9-phenyl-4H-imidazo[1,2-a]indeno[1,2-e]pyrazin-4-one | C19 H11 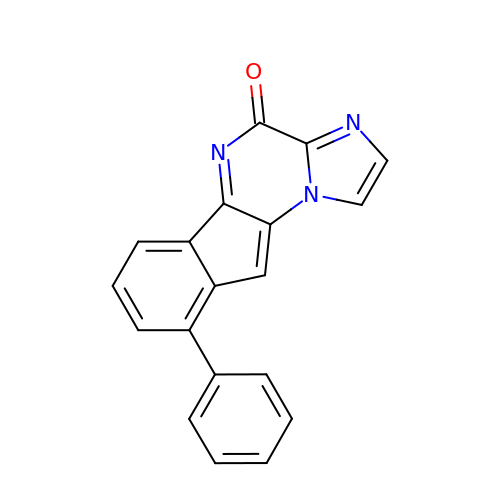N3 O | SFZNDQGUHVYHPD-UHFFFAOYSA-N>INQVRPKLPLLKILHAAGAQGEMFTVKEVMHYLGQYIMVKQLYDAAAQHMVYCGGDLLGELLGRQSFSVKDPSPLYDMLRKNLVT[8x];>XTSFKEYWCLLSPX[8x]

Here we report a novel peptide stapling strategy based on the dithiocarbamate chemistry linking the side chains of residues Lys(i) and Cys(i + 4) of unprotected peptides and apply it to a series of dodecameric peptide antagonists of the p53-inhibitory oncogenic proteins MDM2 and MDMX. In this proof-of-concept study, we firstly used PMI – a potent dodecameric peptide antagonist of MDM2 and MDMX that, despite its high affinity for both proteins, fails to activate p53 and kill p53+/+ tumor cells due presumably to its inability to traverse the cell membrane and susceptibility to proteolytic degradation. Previous structural and functional studies of PMI (TSFAEYWNLLSP) identified Phe3, Trp7 and Leu10 as the most critical residues for MDM2/MDMX binding. Crystallographic studies of peptide–MDM2/MDMX complexes structurally validated the chemoselectivity of the dithiocarbamate staple bridging Lys and Cys at (i, i + 4) positions.

Whereas all 12 residues could be built into each PMI(8,12)-a peptide complexed with MDM2, PMI(4,8)-a was fully defined in only 3 copies of the MDMX complex with no density observed for Ser11 and/or Pro12. In both complexes, however, the crystallographic density for all atoms of the crosslink formed between Lys(i) and Cys(i + 4) unambiguously defined the geometry of the DTC staple. The DTC staple rigidified, at positions (8,12), the C-terminus of PMI in a helical conformation and extended, at positions (4,8), the C-terminal helix of PMI from Leu9 to Ser11. The rigidity of PMI(8,12)-a or PMI(4,8)-a increased to such an extent that the local buried surface area (BSA) slightly decreased as compared with the BSA contributed by PMI to its interface with MDM2/MDMX (Fig. S8†). We deduced the DTC structure of the predominant epimer from the crystal structures of PMI(4,8)-a and PMI(8,12)-a in respective complex with MDMX and MDM2, where Cys8 or Cys12 remained as an l-amino acid residue as shown in the electron density maps.(2E)-3-(3-hydroxy-4-methoxyphenyl)prop-2-enoic 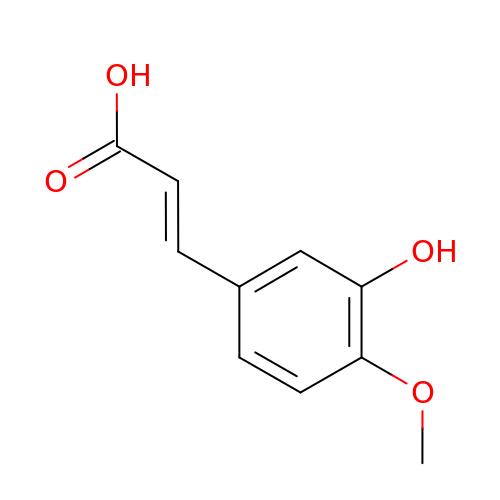acid | C10 H10 O4 | QURCVMIEKCOAJU-HWKANZROSA-N> GPHMKYKLADYRYGREEMLALFLKDNKIPSDLLDK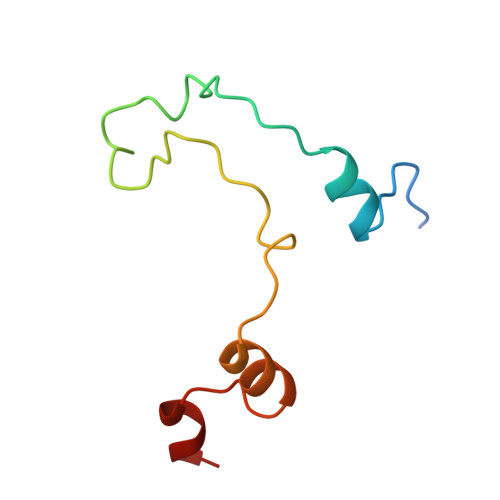EFLPILQEEPLPPLALVPFTEEEQRNFSMSVNSAAVLRLT> MFEARLVQGSILKKVLEALKDLINEACWDISSSGVNLQSMDSSHVSLVQLTLRSEGFDTYRCDRNLAMGVNLTSMSKILKCAGNEDIITLRAEDNADTLALVFEAPNQEKVSDYEMKLMDLDVEQLGIPEQEYSCVVKMPSGEFARICRDLSHIGDAVVISCA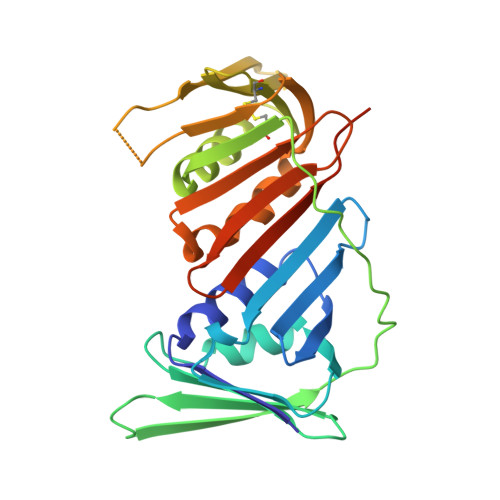KDGVKFSASGELGNGNIKLSQTSNVDKEEEAVTIEMNEPVQLTFALRYLNFFTKATPLSSTVTLSMSADVPLVVEYKIADMGHLKYYLAPKIEDEEGSLEHHHHHH>MKKEVCSVAFLKAVFAEFLATLIFVFFGLGSALKWPSALPTILQIALAFGLAIGTLAQALGPVSGGHINPAITLALLVGNQISLLRAFFYVAAQLVGAIAGAGILYGVAPLNARGNLAVNALNNNTTQGQAMVVELILTFQLALCIFASTDSRRTEPVGSPALSIGLSVTLGHLVGIYFTGCSMNPARSFGPAVVMNRFSPAHWVFWVGPIVGAVLAAILYFYLLFPNSLSLSERVAIIKGTYEPDEDWEEQREERKKTMELTTR[4x]

The flux of water across biological membranes is facilitated by transmembrane protein channels called aquaporins (AQPs). AQP5 is found in tissues such as the lungs, airways and secretory glands and consequently plays a major role in the generation of saliva, tears and pulmonary secretions. There are two consensus PKA sites in AQP5: Ser 156 in cytoplasmic loop D and Thr 259 in the carboxy-terminus; the latter corresponds to Ser 256 in AQP2. Based on the crystal structure of human AQP5 it was hypothesized that phosphorylation of Ser 156 could cause structural changes in loop D that would break its interaction with the carboxy-terminus, thereby flagging the protein for translocation to the plasma membrane.

Finally, we have used x-ray crystallography to show that the phosphomimetic S156E mutation does not cause any significant structural changes to the protein as previously suggested. For full-length AQP5 S156E, additional electron density could be seen beyond Pro 245 in one of the monomers (monomer D), allowing us to build nine more residues. However, this region does not interact with any other residues within the tetramer. Instead, it forms crystal contacts with symmetry-related AQP5 molecules in the crystal packing, explaining why this region is ordered in this particular monomer of the full-length structure. For full-length AQP5 S156E, the limited resolution prevented the identification of water molecules in the channel. In both structures, a lipid molecule could be observed in the central channel formed between monomers in the tetramer, albeit at slightly different positions. Similarly to wild-type AQP5, this lipid was modelled as phosphatidyl serine. We therefore suggest that it is the presence of a phosphate group at Ser 156 rather than a conformational change of the carboxy-terminus that is recognized as a sorting signal, resulting in increased AQP5 membrane abundance.> IQVFLSARPPAPEVSKIYDNLILQYSPSKSLQMILRRALGDFENMLADGSFRAA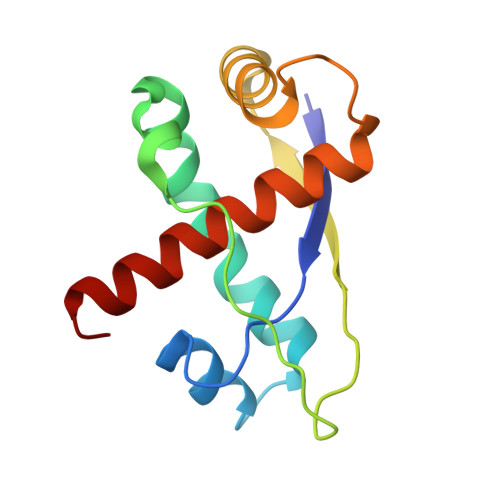PKSYPIPHTAFEKSIIVQTSRMFPVSLIEAARNHFDPLGLETARAFGHKLATAALACFFAREKATNS>KSGKPSGEMDEVGVQKCKNALKLPVLEVLPGGGWDNLRNVDMGRVMELTYSNCRTTEDGQYIIPDEIFTIPQKQSNLEMNSEILESWANYQSSTSYSINTELSLFSKVNGKFSTEFQRMKTLQVKDQAITTRVQVRNLVYTVKINPTLELSSGFRKELLDISDRLENNQTRMATYLAELLVLNYGTHVTTSVDAGAALIQEDHLRASFLQDSQSSRSAVTASAGLAFQNTVNFKFEENYTSQNVLTKSYLSNRTNSRVQSIGGVPFYPGITLQAWQQGITNHLVAIDRSGLPLHFFINPNMLPDLPGPLVKKVSKTVETAVKRYYTFNTYPGCTDLNSPNFNFQANTDDGSCEGKMTNFSFGGVYQECTQLSGNRDVLLCQKLEQKNPLTGDFSCPSGYSPVHLLSQIHEEGYNHLECHRKCTLKVFCKTVCEDVFQVAKAEFRAFWCVASSQVPENSGLLFGGLFSSKSINPMTNAQSCPAGYFPLRLFENLKVCVSQDYELGSRFAVPFGGFFSCTVGNPLVDPAISRDLGAPSLKKCPGGFSQH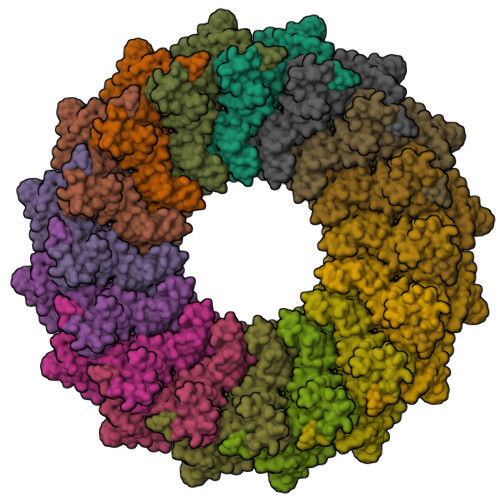PALISDGCQVSYCVKSGLFTGGSLPPARLPPFTRPPLMSQAATNTVIVTNSENARSWIKDSQTHQWRLGEPIELRRAMNVIHGDGGGLSHHHHHH[16x]> EQARPADDALAAL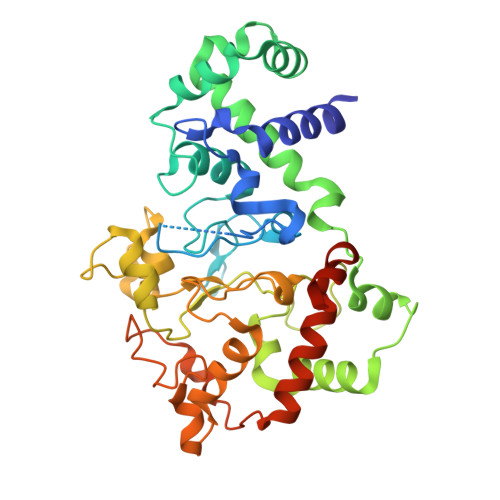GAQLFVDPALSRNATQSCATCHDPARAFTDPREGKAGLAVSVGDDGQSHGDRNTPTLGYAALVPAFHRDANGKYKGGQFWDGRADDLKQQAGQSMLNPVEMAMPDRAAVAARLRDDPAYRTGFEALFGKGVLDDPERAFDAAAEALAAYQATGEFSPFDSKYDRVMRGEEKFTPLEEFGYTVFITWNCRLCHMQRKQGVAERETFTNFEYHNIGLPVNETAREASGLGADHVDHGLLARPGIEDPAQSGRFKVPSLRNVAVTGPYMHNGVFTDLRTAILFYNKYTSRRPEAKINPETGAPWGEPEVARNLSLAELQSGLMLDDGRVDALVAFLETLTDRRYEPLLEESRAAQKDHHHHHH> SNAKNRLGTKALNFTYTLDSGVKGTLYQFPAEYTL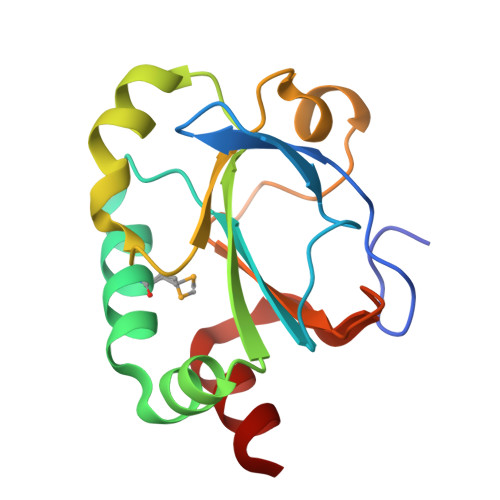LFINNPGCHACAEMIEGLKASPVINGFTAAKKLKVLSIYPDEELDEWKKHRNDFAKEWTNGYDKELVIKNKNLYDLRAIPTLYLLDKNKTVLLKDATLQKVEQYLAE>[2x]GSHMFSCVKPYEDQNYSALRRDCRRRKVLFEDPLFPATDD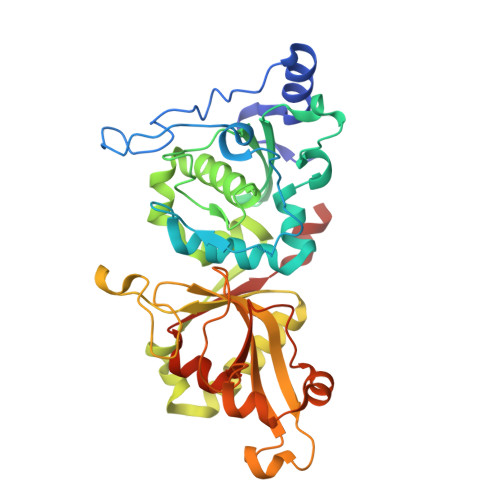SLYYKGTPGPAVRWKRPKGICEDPRLFVDGISSHDLHQGQVGNCWFVAACSSLASRESLWQKVIPDWKEQEWDPEKPNAYAGIFHFHFWRFGEWVDVVIDDRLPTVNNQLIYCHSNSRNEFWCALVEKAYAKLAGCYQALDGGNTADALVDFTGGVSEPIDLTEGDFANDETKRNQLFERMLKVHSRGGLISASIKAVTAADMEARLACGLVKGHAYAVTDVRKVRLGHGLLAFFKSEKLDMIRLRNPWGEREWNGPWSDTSEEWQKVSKSEREKMGVTVQDDGEFWMTFEDVCRYFTDIIKCRVILENLYFQGHHHHH> METKL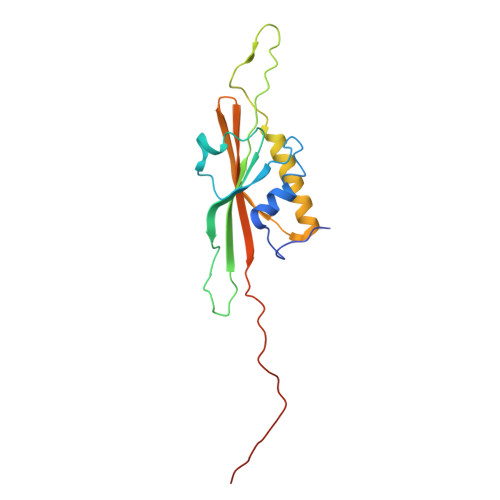KLTYSNRLTLPEIAKHIVSPTFHELEGRAIPVTGVEDDKEGQSAITKPFALVGLRIGDTSGPAEIGENSRINLRDDFIIEFNFNKDRYKKGGAETSLFSYYDYESIRDRLFNAMVAFAGEYGITFEFVSLDISTEGDTVYIEFRFRQNFDWCEADRESDTVIKAGSFSLNLKGC>[2x]MSFEGKIALVTGASRGIGRAIAETLVARGAKVIGTATSENGAKNISDYLGANGKGLMLNVTDPASIESVLENIRAEFGEV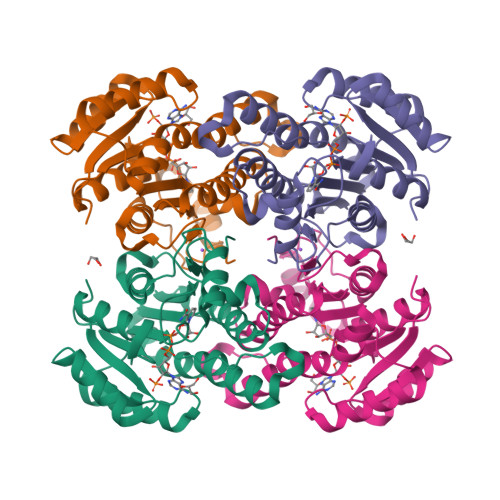DILVNNAGITRDNLLMRMKDDEWNDIIETNLSSVFRLSKAVMRAMMKKRCGRIITIGSVVGTMGNAGQANYAAAKAGLIGFSKSLAREVASRGITVNVVAPGFIETDMTRALSDDQRAGILAQVPAGRLGGAQEIASAVAFLASDEASYITGETLHVNGGMYMV> GSELNTERQIFLEACIVRIMKAKRNLPHTTLVNECIAQSHQRFNAKVSMVKRAIDSLIQ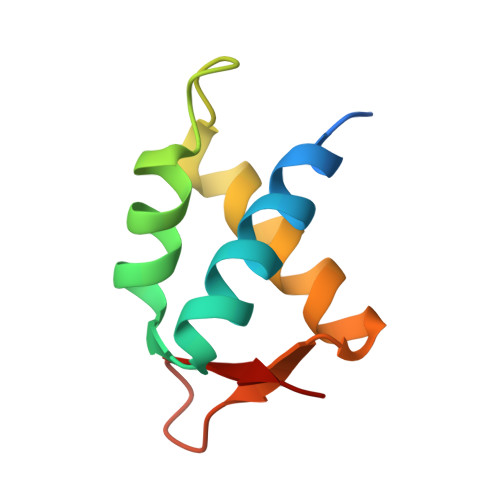KGYLQRGDDGESYAYLA>MTNQKFFTLSNGNKIPAVAVVGTGTKWAHAEETDATFSQELTDIVKLSLDTVPGIVHIDAAETYKTYPELGAALKETKKPREEIFITDKFSSLHKISEDPKSALETALNKLGVDYVDLYLIHSPFFDKDLNIDLETAWKQLEELYKSGKAKNIGVSNFTVEDLKKVLAIAEIKPQVNQIEFSPFLQNQTPGIVEFSQKNDILLEAYSPLGPLQKKPTDADQQPFYQYLKELSEKYNKTEAQVLLLWVYKRGILPVTTSAKIERIKQAQD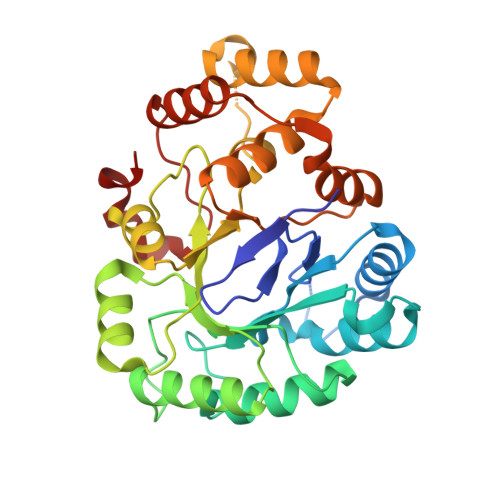IFSFDLTEEEVKKITDLGLQHEPVRLWHVDFYTKYNSEAQK[4x]> MSNFKVRDPVIQERLDHDYAHHPLVARMNTLDQGNMSQAEYLVQKRHYLVFLIAHHYYEAYLRRMGGIQRRDHLQTLRDQKPRERADRVSAASAYDAGTFTVPSRPGP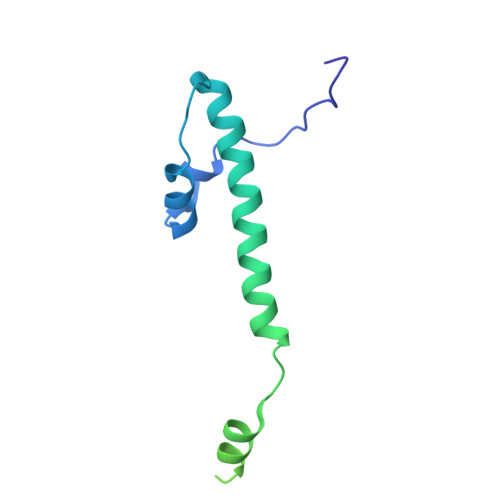ASGTTPGGQDSLGVSGSSITTLSSGPHSLSPASDILTTLSSTTETAAPAVADARKPPSGKKK>SEKPVYLSVKADNSMFIGNDPVTDETMITALNALTEGKKDTTIFFRADKTVDYETLMKVMDTLHQAGYLK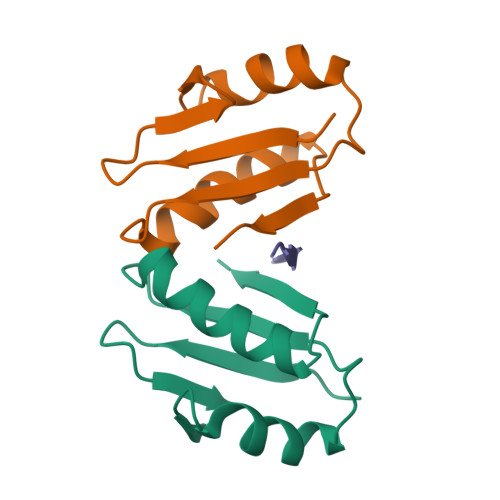IGLVGEETAKAK[2x];> KKAQPISVTMVTPADLEPPQAKK(5E,14E)-11-oxoprosta-5,9,12,14-tetraen-1-oic acid | 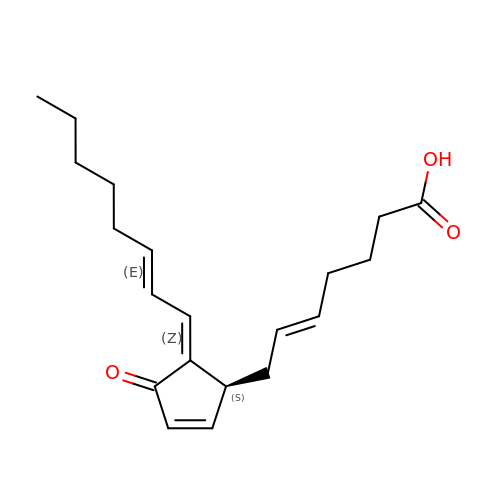C20 H28 O3 | VHRUMKCAEVRUBK-XOVNXQNQSA-N> MAWSHPQFEKSAAKENTQQKEIKRQPAVELAVFNLNSVTDVADLQMIASQVQLYLQVCGNTTLEQIKSKANITTVANIFALTGSVLDLMLYATDKKTGDAAVQRGALLAANLIGLFSEPNNEAHARMALRPMFGLMAECLYRENGKIKETDIKRLGLHLNAMIAGDLENFLKETQAKLSSLLISATTLGVTILQSMATPATGINAGITTAAGASAEKRDPKLKFTNWAVPLIDLLGKPSQANLTPKIQPNITSRLQQEATQAIAALSQTLQQQANA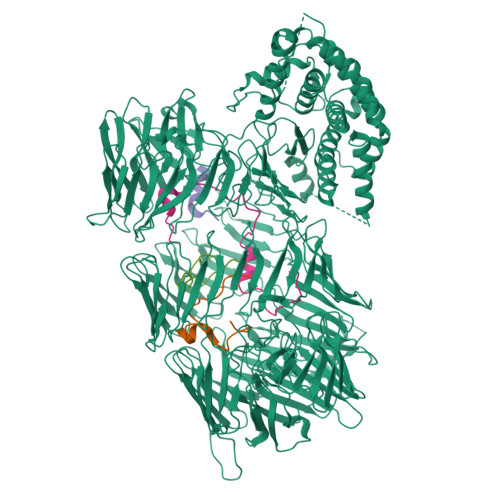GQKYTLAWLLQETLKAIQALENKGNASVPINQTGEYERHTKGDTLEFVSLQADALNAPPCEGADSQSGKSISYSIGAERVQHADFYLPKIGFSFIRQYNSQMDEFDQSMVGARWMMPFSNMIQQNAQGYLFIDSKGRKHQLPVSIIFETYEVPYEGWIIKPLKNGELILDFGGEWRSHFQSFDGGKNYYLVKKMNETSQEEILLEYLLLDHIAYLKVINFKLKQAEYELKFAFNEQVKIIAVFLDDKAEPLARYEYDTQGNLIKAIDQNGHTRTYEYNQFHQLTRYTDRTGRGQNIRYESTEAKAKAIEEWADDGSFHTKLKWHPRLRQVAVYDAYDVPTYYYFDLDGFTYRTRLADGRESWYSRDGKKRITRQIDFDGRETQQEYNDQDQLVKIVQPNGGIIRFAYNKQGNLVEIKDPEGSIWKREYDENRNVSKEINPLGHITQYKYNNDNQLVEVIDAKGGVKKIQYNELGQMISYTDCSGKSSTWEYDEDGALTAEQTANNKVVQYFYSTKGRDKGQLQSIIYPDGLKEYFEHDEEGRLLKHTDTKGLVTEYKYNQVGLLEQRIDANRHSVAYQWDKQGRIQKLINQNQAEYLFGYNPYGYLIREQAFDGEEKHYSYNENGRLFQIRRPNILTQFDYYADGQIASKSFTHLHTGQKQTEQFDYNLNSQLSRASNEVSQIDLYRNALGQLVREHQHYKIPELKPLTAVLHYEYDELGNLIKTIRPDGHTLNHLVYGSGHIYAIGLNNQEVVSFQRDDLHRETTRLLANGLMQTKQYNDVGLLSSQFIQPEQETQDYLQYQAHRKYHYDKNYLLSQVEDSRLGKLNYQYDPIGRLIAAQSLHKTESFNFDPAGNLIDSESVLSPAQIKNNLIKSYKGKHYQYDVQGNVTEIIQAGKNLKLTWDNQNRLIRSDNNGLVTEYGYDVFGRRLYKKTAKELTLFGWDGDLMIWESFKSAQTNYTKHYIYEPDSFVPLLQAGYKDFIQLIETPDYQEYQTKPYSIYKDPVWNRNLGKERTALEQFTFYHCDQVGTPQTMTNIRGECVWEILQDTWGAVSQIKALNQDNPFEQNNLRFQGQYYDRETELHYNRYRYYEPHSARYVSKDPIGLEGGMNTSSYVSDPNQWIDPKGLNSFNYGEMFGIPASAQSGLAYQGQRNYECYAETGELCKIKVPPLFDYVACSGGGLGIGVGFVKNQWTGEYYISGSKDSLLIPVAKSVAQNKQFSAKDLAGASCVGGNIHNIPSYTKTTMTMGEITNEFVSGASVTVGGGAYGAVANVVVPLVSKSSPVKGTWASELGVGTPGFNVGVSGTVSVDTILDAVKPSKKHHHHHH> GSHMASDLLELTEDMEKEISNALGHGPQDEILSSAFKLRITRGDIQTLKNYHWLNDEVINFYMNLLVERNKKQGYPALHVFSTFFYPKLKSGGYQAVKRWTKGVNLFEQEIILVPIHRKVHWSLVVIDLRKKCLKYLDSMGQKGHRICEILLQYLQDESKTKRNSDLNLLEWTHHSMKPHEIPQQLNGSDSGMFTCKYADYISRDKPITFTQHQMPLFRKKMVWEILHQQLL;> MANDHINLKVAGQDGSVVQFKIKRHTPLSKLMKAYCERQGLSMRQIRFRFDGQPINETDTPAQLEMEDEDTIDVFQQQTGG;> SLNTGEPAPVLSSPPPADVSTFLAFPSPEKLLRLGPKSSVLIAQQTDTSDPEKVVSAFLKVSSVFKDEATVRMAVQDAVDALMQKAFNSSSFNSNTFLTRLLVHMGLLKSEDKVKAIANLYGPLMALNHMVQQDYFP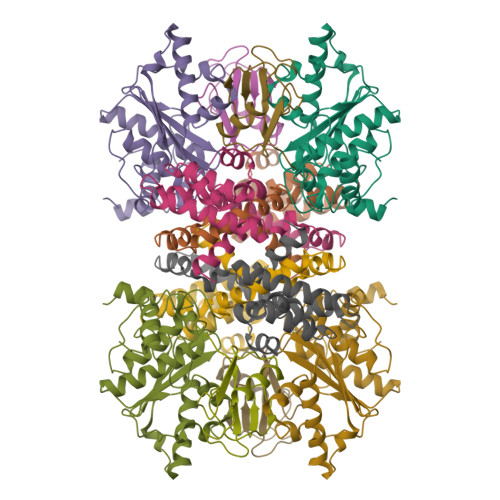KALAPLLLAFVTKPNSALESSSFARHSLLQTLYKV>MTRRIRIGGAQMGAISRSDSKKEIVDRLIALLRQASEKGCELVVFPELALSTFFPRWYAERDGMDGYFEDGMPNAATLPLFEEARRLGIGFSLGYAELVQEDGRVRRFNTTVLVERNGEIVGKYRKIHLPGHAEYEPERSHQHLEKRYFEVGNTGFQVWDAFGGRVGMAICNDRRWVETYRVMGLQDVELILIGYNTPVADSLSGESETLRMFHNHLTMQAGAYQNSTWVVGVAKAGVEDGHRLMGGSVIVAPTGEIVAQAMTEGDELIVADCDLDRCRYYKSHIFNFAAHRRPEFYQRI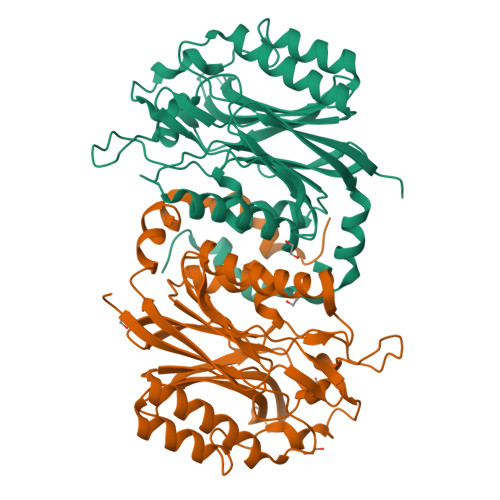TSQTGVE[2x]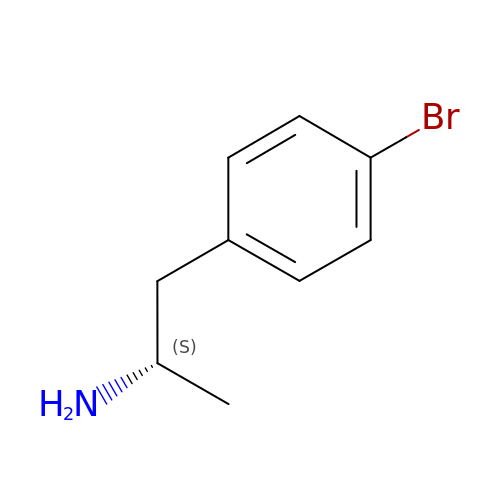(2S)-1-(4-bromophenyl)propan-2-amine | C9 H12 Br N | SMNXUMMCCOZPPN-UHFFFAOYSA-N> MVKLKSIQELENLREKIKEAKKKEKIVIRICGGTGCRASGSLAVRDELVKVLKREGFANVDVNLSSDCLENTSEVHVKMTGCQGFCAQGPLMTIEPLGVFYVGVKPEDVEEIVEKSIKKNEIIERLLYHDPATGKTYVKRDENPFYAKQTRLVLKHCGTVDPASVYDYIAEGGYSAIAKALTMDRKQIIDEVIKSGLRGRGGAGFPTGEKWLGAYKNQSPKKYIICNGDEGDPGAFMDRSVMEGDPHKVIEGMMIGAYAIGSDEGYIYVRAEYPLAVQMLRKAIEECEKLGLLGDNILGTGFSFRLHVREGAGAFVCGESTALTYSIEGKRGMPRVRPPRTNECGLWEMPTVLNNVETFACIPEIILNGGEWFASIGTPTSTGTKIFALSGKVNRTGLVEVPMGLKLRELIFDIGGGIANNKKFKAVQLGGPSGGCVPESQLDLPIDFDSLSKAGAIMGSGGVVVVDEDTCMVDFA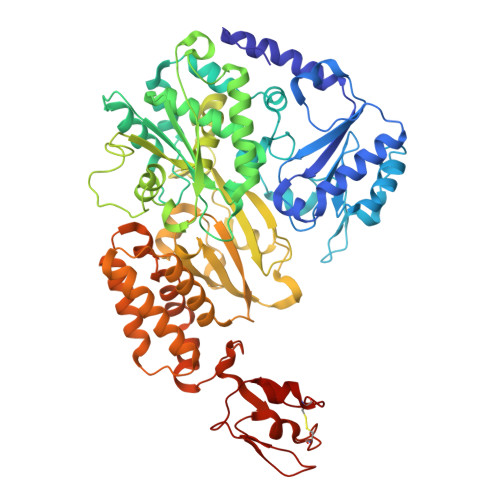KFFTNFIVEESCGKCIPCREGNKKMLEILERITEGKGKEGDIELLEELGDVIISASLCGLGKTAPNPVLSTIKHFRDEYEAHIRDKKCPAGACQALAAYKIDPGKCIGCGKCVKVCPVGAISGEKKKPHVIDQSKCIKCGACAENCPKGAIYKG>[3x]MDDDGTGQKQIWRIEGSNKVPVDPATYGQFYGGDSYIILYNYRHGGRQGQIIYNWQGAQSTQDEVAASAILTAQLDEELGGTPVQSRVVQGKEPAHLMSLFGGKPMIIYKGGTSREGGQTAPASTRLFQVRANS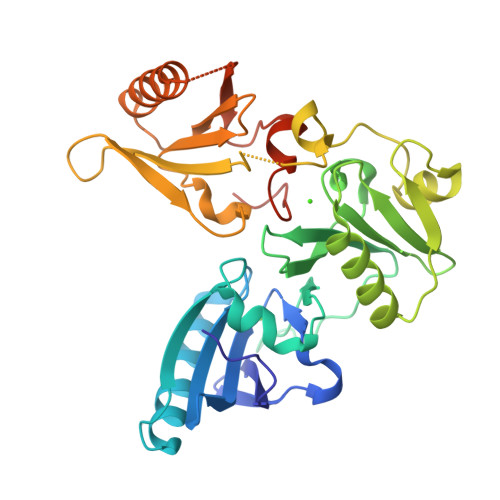AGATRAVEVLPKAGALNSNDAFVLKTPSAAYLWVGTGASEAEKTGAQELLRVLRAQPVQVAEGSEPDGFWEALGGKAAYRTSPRLKDKKMDAHPPRLFACSNKIGRFVIEEVPGELMQEDLATDDVMLLDTWDQVFVWVGKDSQEEEKTEALTSAKRYIETDPANRDRRTPITVVKQGFEPPSFVGWFLGWDDDYWSVDPLDRAMAELAA(3R)-3-({(4-aminobenzyl)[(4-aminophenyl)acetyl]amino}methyl)-5-(hydroxymethyl)-2,3,4,7-tetrahydro-1H-azepinium 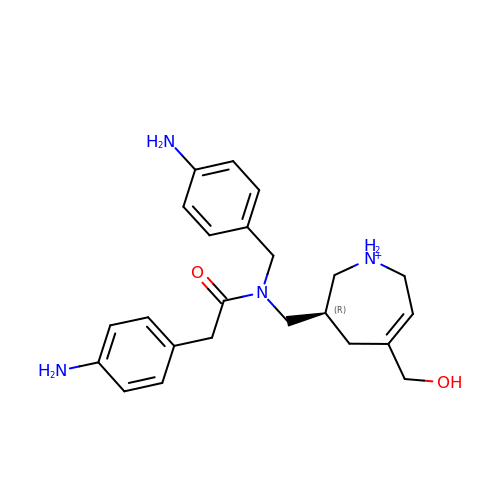| C23 H31 N4 O2 | WRSLWDODYIRHLE-HXUWFJFHSA-O>GMIRLLYLLVKPAGMSDETFRAECLRHYEMSHDVPGLHKYEVRLVAEQPTDTHVPFFDIGHVDAIGECWFKDDAAYATYMASDIRKAWFEH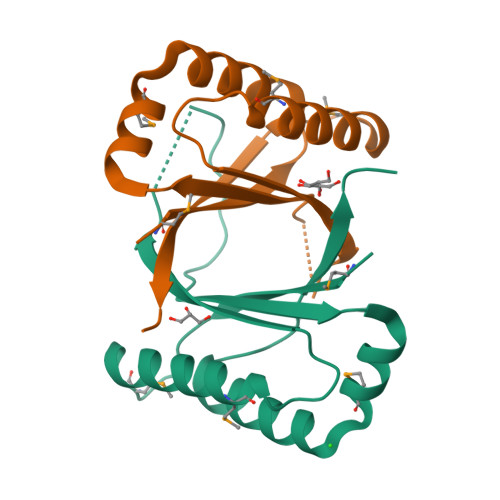GKTFIGQLKPFRTAPVAGDEPAS[2x]>GGSMSKSKVDNQFYSVEVGDSTFTVLKRYQNLKPIGSGAQGIVCAAYDAVLDRNVAIKKLSRPFQNQTHAKRAYRELVLMKCVNHKNIISLLNVFTPQKTLEEFQDVYLVMELMDANLCQVIQMELDHERMSYLLYQMLCGIKHLHSAGIIHRDLKPSNIVVKSDCTLKILDFGLARTAGTSFMMTPYVVTRYYRAPEVILGMGYKENVDIWSVGCIMGEMVRHKILFPGRDYIDQWNKVIEQLGTPCPEFMKKLQPTVRNYVENRPKYAGLTFPKLFPDSLFPADSEHNKLKASQARDLLSKMLVIDPAKRISVDDALQHPYINVWYDPAEVEAPPPQIYDK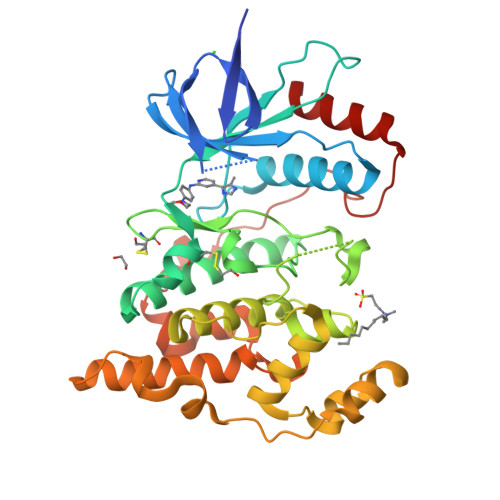QLDEREHTIEEWKELIYKEVMNSE[4x]> MGSSHHHHH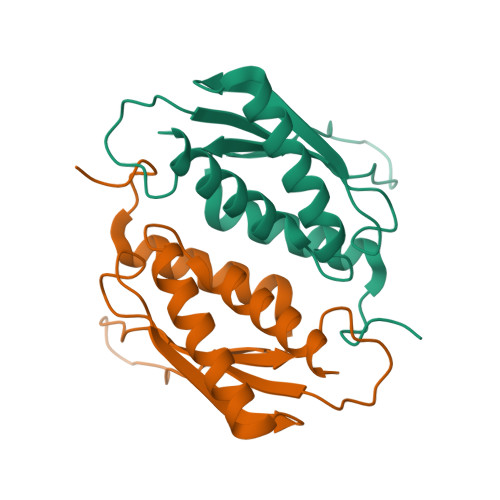HSGESYPQRQDHELQALEAIYGADFQDLRPDACGPVKEPPEINLVLYPQGLTGEEVYVKVDLRVKCPPTYPDVVPEIELKNAKGLSNESVNLLKSRLEELAKKHCGEVMIFELAYHVQSFLSEHNK>[2x]SNAMAKNKLLRMDNVSIVVESLDNAISFFEEIGLNLEGRANVEGEWAGRVTGLGSQCVEIAMMVTPDGHSRIELSRFLTPPTIADHRTAPVNALGYLRVMFTVEDIDEMVSRLT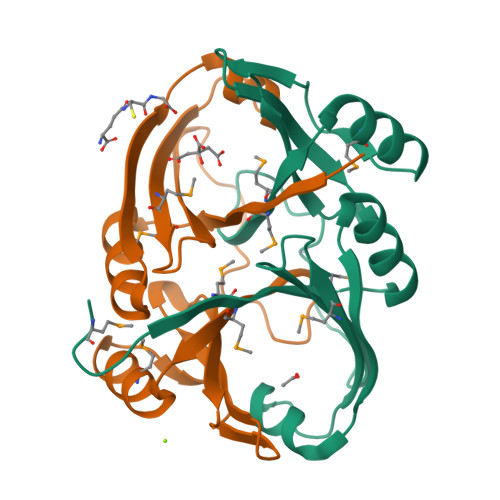KHGAELVGEVVQYENSYRLCYIRGVEGILIGLAEELGNK>SGGGMLTLIQG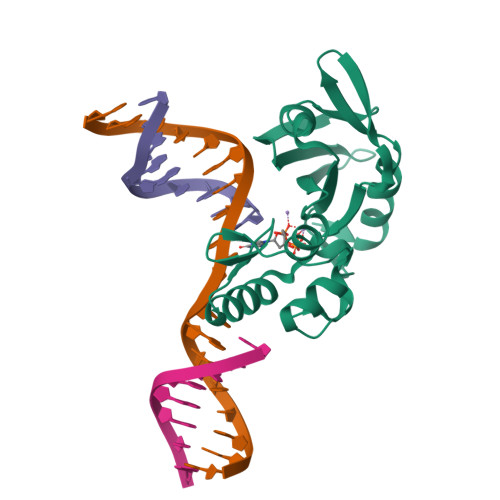KKIVNHLRSRLAFEYNGQLIKILSKNIVAVGSLRREEKMLNDVDLLIIVPEKKLLKHVLPNIRIKGLSFSVKVCGERKCVLFIEWEKKTYQLDLFTALAEEKPYAIFFFTGPVSYLIRIAAALKKKNYKLNQYGLFKNQTLVPLKITTEKELIKELGFTYRIPKKRL[2x]> SKPIILRFNQ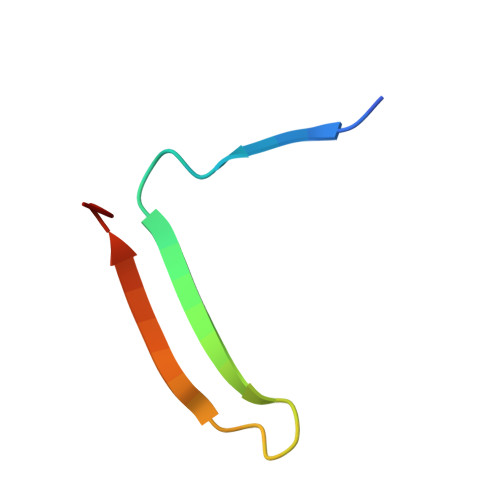PFIIMIFDHFTWSSLFLARVMNPV>MYTLNWQPPYDWSWMLGFLAARAVSSVETVADSYYARSLAVGEYRGVVTAIPDIARHTLHINLSAGLEPVAAECLAKMSRLFDLQCNPQIVNGALGRLGAARPGLRLPGCVDAFEQGVRAILGQLVSVAMAAKLTARVAQLYGERLDDFPEYICFPTPQRLAAADPQALKALGMPLKRAEALIHLANAALEGTLPMTIPGDVEQAMKTLQTFPGIGRWTANYFALRGWQA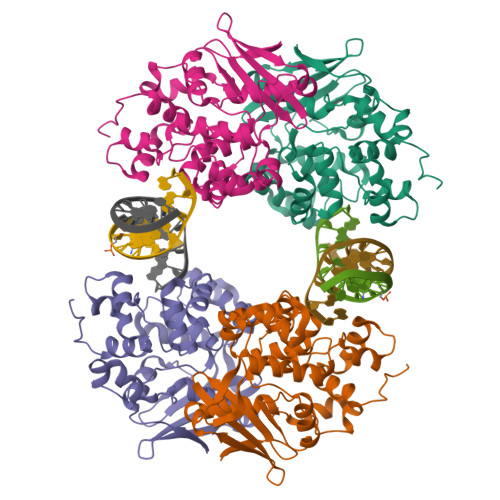KDVFLPDDYLIKQRFPGMTPAQIRRYAERWKPWRSYALLHIWYTEGWQPDEA[4x]>[2x]MYGKGKSNSSAVPSDSQAREKLALYVYEYLLH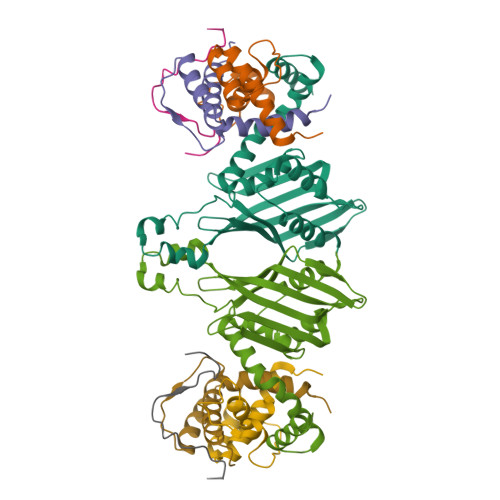VGAQKSAQTFLSEIRWEKNITLGEPPGFLHSWWCVFWDLYCAAPERRETCEHSSEAKAFHDY;> YTEFAPPPTPMVDHLVASNPFEDDFGA;> GIGRHTPYGNQTDYRIFELNKRLQNWTEECDNLWWDAFTTEFFEDDAMLTITFCLEDGPKRYTIGRTLIPRYFRSIFEGGATELYYVLKHPKEAFHSNFVSLDCDQGSMVTQHGKPMFTQVCVEGRLYLEFMFDDMMRIKTWHFSIRQHRELIPRSILAMHAQDPQMLDQLSKNITRCGLSNSTLNYLRLCVILEPMQELMSRHKTYSLSPRDCLKTCLFQKWQRMVAPP> NAVVRSSPGIYSNCFSLRAPLKPDGPKSFTCDLMGGGVVTDGDTGWQVTVRNTPVSNLL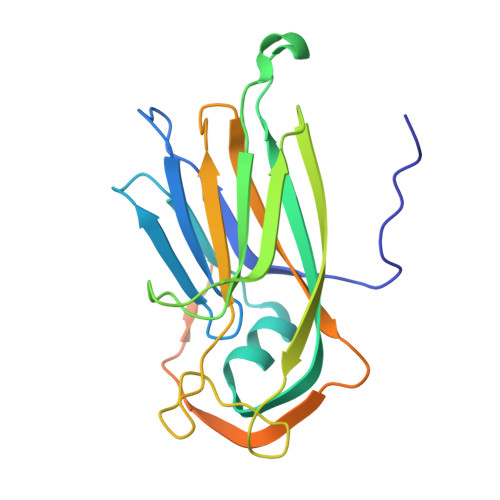RTAAWKRGTVHVQVVLAGASVKRSDWDSTVQIFLRQSMATSSYDAKIWDICQPGAAMLEFSFDVVGPNSGFEMWDSNWASQTSWFLEFLISNPAQNTLFEVNLRLDENFSVAGTTLMPPFVLDRVSVARPLLGKQTKTVARSARVVRETKEASESP> MSTPTGSRRIFSGVQPTSDSLHLGNALGAVAQWVGLQDDHDAFFCVVDLHAITIPQDPEALRRRTLITAAQYLALGIDPGRATIFVQ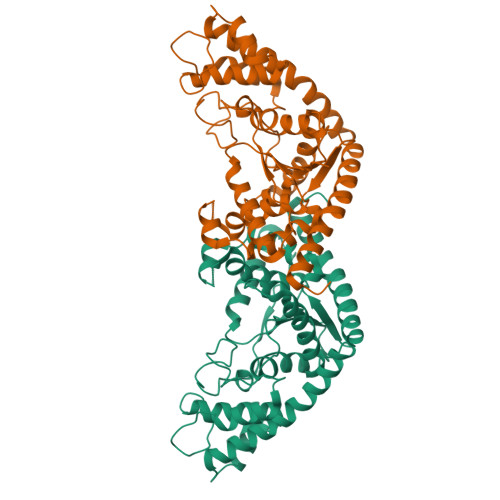SQVPAHTQLAWVLGCFTGFGQASRMTQFKDKSARQGSEATTVGLFTYPVLQAADVLAYDTELVPVGEDQRQHLELARDVAQRFNSRFPGTLVVPDVLIPKMTAKIYDLQDPTSKMSKSAGTDAGLINLLDDPALSAKKIRSAVTDSERDIRYDPDVKPGVSNLLNIQSAVTGTDIDVLVDGYAGHGYGDLKKDTAEAVVEFVNPIQARVDELTADPAELEAVLAAGAQRAHDVASKTVQRVYDRLGFLLLEHHHHHH> SADIDECESSPCINGVCKNSPGSFICECSSESTLDPTKTICIETIKGTCWQTVIDGRCEININGATLKSQCCSSLGAAWGSPCTLCQVDPICGKGYSRIKGTQCEDIDECEVFPGVCKNGLCVNTRGSFKCQCPSGMTLDATGRICL

The fibrillins and latent transforming growth factor-β binding proteins (LTBPs) form a superfamily of structurally-related proteins consisting of calcium-binding epidermal growth factor-like (cbEGF) domains interspersed with 8-cysteine-containing transforming growth factor β-binding protein-like (TB) and hybrid (hyb) domains. Fibrillins are the major components of the extracellular 10–12 nm diameter microfibrils, which mediate a variety of cell-matrix interactions. The molecular organization of the fibrillins, and the related LTBPs, is dominated by calcium-binding epidermal growth factor-like (cbEGF) domains. Related domains, the hybrid (hyb) domains, which have sequences similar to both the TB and cbEGF domains, are found near the N termini of these molecules, with two being found in each of the fibrillins (Corson et al., 2004; Pereira et al., 1993; Zhang et al., 1994), and one in each of the LTBPs (Gibson et al., 1995; Giltay et al., 1997; Kanzaki et al., 1990; Yin et al., 1995).

Here we present the X-ray crystal structure of a cbEGF9-hyb2-cbEGF10 triple domain fragment from fibrillin-1, providing the first high-resolution structure of a hyb domain found in the fibrillin/LTBP protein family. Crystals were grown in the presence of 20 mM CaCl2 in order to saturate the N-terminal cbEGF9 Ca2+ binding site, which is likely to have a relatively low affinity for Ca2+ based on previous work (McGettrick et al., 2000; Smallridge et al., 1999, 2003). The overall shape of cbEGF9-hyb2-cbEGF10 resembled the tetragonal pyramidal shape previously seen in the fibrillin-1 cbEGF22-TB4-cbEGF23 structure (Lee et al., 2004), with slightly smaller dimensions of approximately 6.5 × 3.5 × 2.5 nm. Like the TB4 fragment, extensive interdomain contacts were observed between cbEGF9 and hyb2, and between hyb2 and cbEGF10. As expected, both of the cbEGF domains in the structure were found to contain bound Ca2+. In cbEGF9, Ca2+ was coordinated by three side-chain oxygens (Asp807, Glu810, and Asn823), three main-chain carbonyls (Ile808, Ser824, and Ser827), and a single water molecule. Coordination of the Ca2+ in cbEGF10 was through interactions with three side-chain oxygens (Asp910, Glu913, and Asn928), three main-chain carbonyls (Ile911, Thr929, and Ser932), and a single water molecule. We show that these highly disulphide-bonded domains are structurally related to both the TB and EGF domains, as suggested by previous sequence data (Corson et al., 1993; Pereira et al., 1993), with an N-terminal region containing a hydrophobic core consisting of a conserved tryptophan as in the TB domains (Lee et al., 2004; Yuan et al., 1997), and the C-terminal region containing a disulphide-stabilized β sheet similar to some EGF domains (Knott et al., 1996). The hyb2 structure shows a rearrangement of disulphides toward the C-terminal part of the domain so that the cysteine corresponding to C8 in the TB domain forms a disulphide bond with the second to last residue of the domain.>GSGGSIRLADLAQQLDAELHGDGDIVITGVASMQSAQTGHITFMVNPKYREHLGLCQASAVVMTQDDLPFAKSAALVVKNPYLTYARMAQILDTTPQPAQNIAPSAVIDATAKLGNNVSIGANAVIESGVELGDNVIIGAGCFVGKNSKIGAGSRLWANVTIYHEIQIGQNCLIQSGTVVGADGFGYANDRGNWVKIPQIGRVIIGDRVEIGACTTIDRGALDDTIIGNGVIIDNQCQIAHNVVIGDNTAVAGGVIMAGSLKIGRYCMIGGASVINGHMEI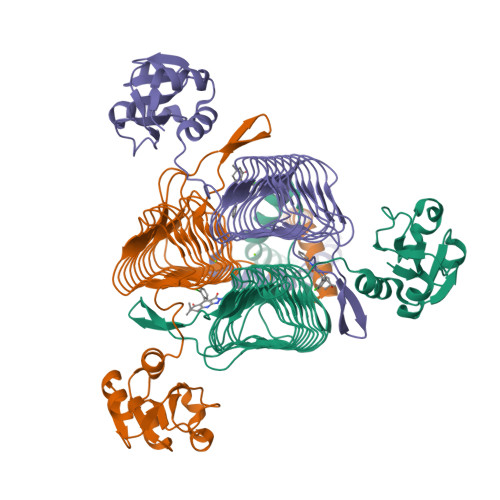CDKVTVTGMGMVMRPITEPGVYSSGIPLQPNKVWRKTAALVMNIDDMSKRLKSLERKVNQQD[3x]> MEGQGCCGGGGGKTEMIPTEEALRIVFGVSKRLPPVIVSLYEALGKVLAEDIRAPDPLPPYPASVKDGYAVVASDGPGEYPVITESRAGNDGLGVTVTPGTVAYVTTGGPIPDGADAVVQVEDTKVIGDVSTESKRVKILIQTKKGTDIRRVGCDIEKDATVLTTGERIGASEIGLLATAGVTMVKVYPMPIVAILSTGDELVEPTAGTLGRGQIRDSNRAMLVAAVMQQQCKVVDLGIVRDDRKELEKVLDEAVSSGVDIILT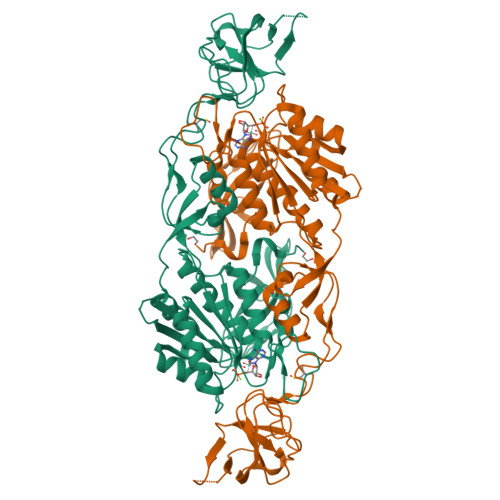SGGVSMGDRDFVKPLLEEKGKVYFSKVLMKPGKPLTFAEIRAKPTESMLGKTVLAFGLPGNPVACLVCFNIFVVPTIRQLAGWTSPHPLRVRLRLQEPIKSDPIRPEFHRAIIKWKDNDGSGTPGFVAESTGHQMSSRLLSMRSANALLELPATGNVLSAGSSVSAIIVSDISAFSIDKKASLSEPRSWSHPQFEK>MLSPKAATLAERSAGLAFSLYQAMAKDQAVENILLSPVVVASSLGLVSLGGKATTASQAKAVLSAEQLRDEEVHAGLGELLRSLSNSTARNVTWKLGSRLYGPSSVSFAEDFVRSSKQHYNCEHSKINFRDKRSALQSINEWAAQTTDGKLPEVTKDVERTDGALLVNAMFFKPHWDEKFHHKMVDNRGFMVTRSYTVGVTMMHRTGLYNYYDDEKEKLQIVEMPLAHKLSSLIILMPHHVEPLERLEKLLTKEQLKIWMGKMQKKAVAISLPKGVVEVTHDLQKHLAGLGLTEAIDKNKADLSRMSGKKDLYLASVFHATAFEWDTEGNPFDQDIYGREELRSPKLFYADHPFIFLVRDTQSGSLLFIGRLVRPKGDKMRDELLEHHHHHH[2x];>[6x]XPPGPPGPPGPRGFPGPPGPPG

In order to function, collagens require the specific chaperone HSP47 for proper folding and secretion. Proper triple-helix formation as well as exit from the ER of procollagen molecules depends critically on HSP47, an ER-resident chaperone belonging to the serpin family. The interaction involves Gly-Xxx-Arg triplets exclusively on triple-helical procollagen. The arginine residue is located in the so-called Y0 position and forms a crucial salt bridge with an aspartic acid of HSP47 (16).

To explain this observation, we determined cocrystal structures of HSP47 with synthetic model peptides containing the GPRGFP and GPRGLP motifs (from here on called RGF and RGL, respectively). The complexes of HSP47:CMP[RGF/RGL] crystallized in space groups P3221 and I222, respectively, which both are different from those of all previously determined HSP47 crystal structures. The structures were refined at resolutions of 1.94 Å and 2.5 Å with refinement statistics of R/Rfree 20.3/24.8% and 21.3/26.7%. In contrast to all those RGP structures, these new ones employing the RGL and RGF collagen model peptides have only the A-site occupied by HSP47. To adapt the bulky hydrophobic side chains at the X+1 position, conformational rearrangements of HSP47 take place. In both structures, the loop containing His274 moves slightly outward by approximately 1.8 Å (Cα – Cα distance). For the phenylalanine-containing triple helix, Met225 switches to a different rotamer to form a small pocket shielding the phenylalanine from the solvent. In the RGF complex, the bound HSP47 at the A-site recognizes the arginine from the trailing chain and buries the phenylalanine from the middle strand. The results were similar to the prediction mentioned before (RGF/B and RGL/B), the phenylalanine and—less prominently—the leucine side chain clash with either the modeled second HSP47 molecule or the collagen backbone.> RSVAETPTYPWRDAETGERLVCAQCPPGTFVQRPCRRD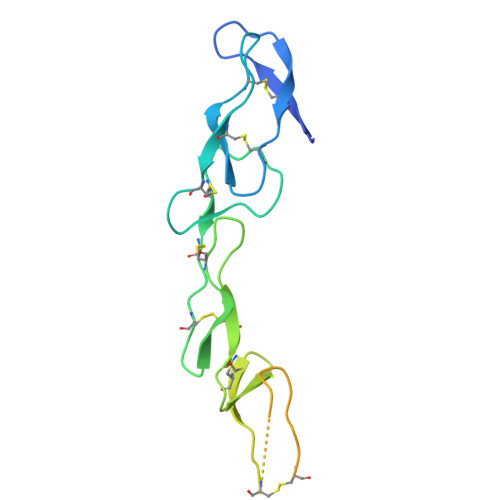SPTTCGPCPPRHYTQFWNYLERCRYCNVLCGEREEEARACHATHNRACRCRTGFFAHAGFCLEHASCPPGAGVIAPGTPSQNTQCQPCPPGTFSASSSSSEQCQPHRNCTALGLALNVPGSSSHDTLCTSTGHHHHHH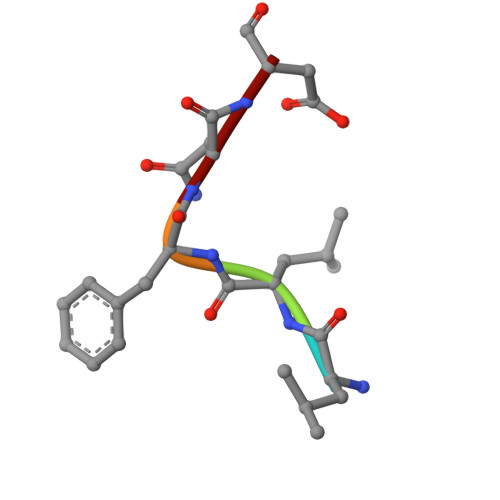> LLFND> MVYTRWKCDRLPVFQLKLFTQEYPMHAAVGIFTIIFLWKHMSHCSEETERKYGWWAGYPYWRDPIARRNETKYKQMIINNDVDITHPKWTGCSVEQL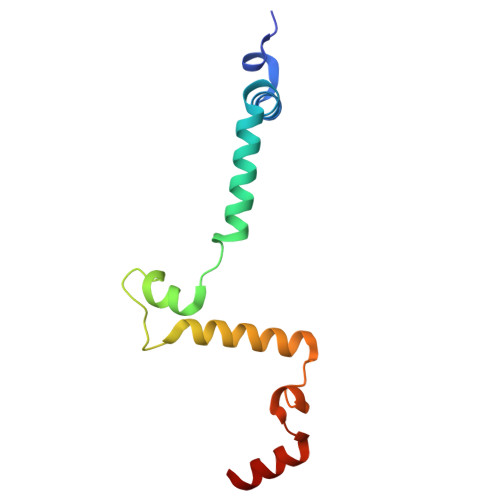EELSRVV2-[2-[(4-oxidanylidene-3~{H}-quinazolin-2-yl)sulfanyl]ethanoylamino]thiophene-3-carboxamide | C15 H12 N4 O3 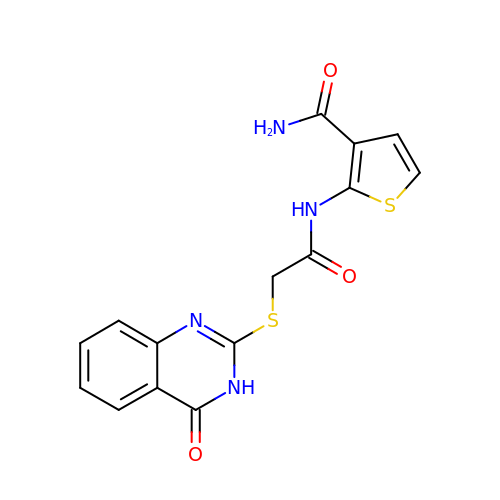S2 | ZSLPDQIUTTUTDY-UHFFFAOYSA-N>MQQKLENIKFVITDVDGVLTDGQLHYDANGEAIKSFHVRDGLGIKMLMDADIQVAVLSGRDSPILRRRIADLGIKLFFLGKLEKETACFDLMKQAGVTAEQTAYIGDDSVDLPAFAACGTSFAVADAPIYVK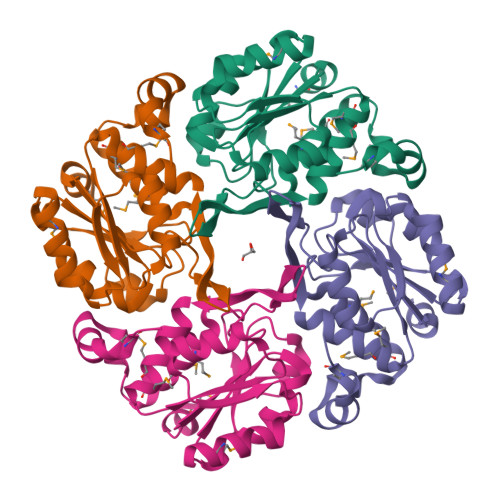NAVDHVLSTHGGKGAFREMSDMILQAQGKSSVFDTAQGFLKSVKSMGQ[4x]>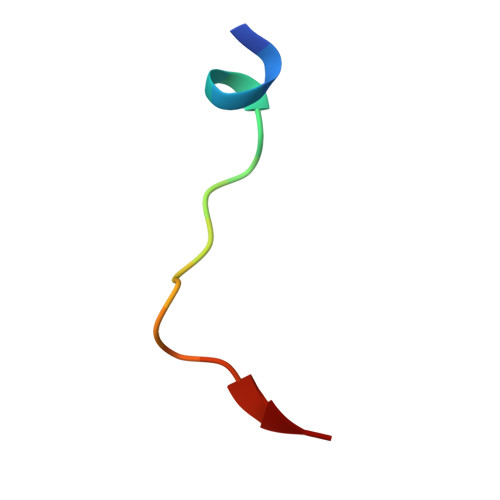 DLEMLAPYIPMDDDFQL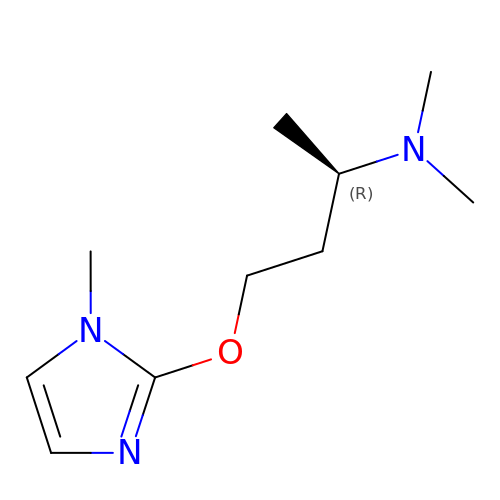(2R)-N,N-dimethyl-4-(1-methylimidazol-2-yl)oxy-butan-2-amine | C10 H19 N3 O | VPQCJEWNIYWNLE-SECBINFHSA-N> MKKILIVSFLGKGRYYETFYYSIEHSEKMVKKRLSPLANAILEKENGNDVEIIFFVTNEVKNEFLYDENNEYAKNILNELNEIKNYGIKVSYRDIPKGKNYEELEIIMEEIEKLLLDFKGNKVIFDLTHGLR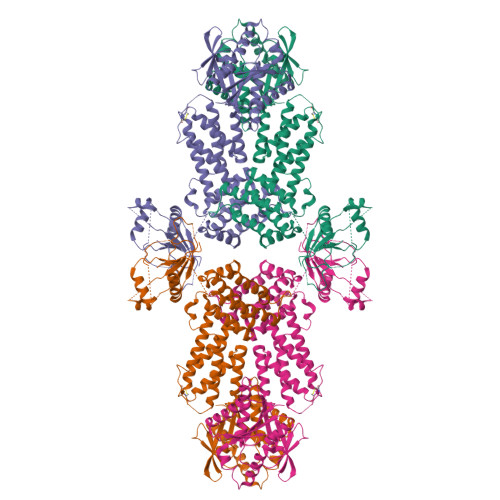HMAIFTSSTVFYFKNLMEKANKLEMKIVYGAYEIGEEIEKNLKKVPILDITQTLELSDLTIALEEFERYGITERMIIVLKNIQKIVAKNKLCNLNELKFSSLSRELKLFEELLKIPSPPEKIANSIYKINDILESSIREFKLCSKNSENLFFIKPIQKFLVDFQKIVLEKLPLDKKINKYSNIATLEKVEFMKNIIKLLINWKMYSEAVIHLRELLIDIKLIENGKYFYYNNKDFREKYWMYSYNIVDTKDKELPKKIEELLKNVKGWRNSVAHGGRANTSINQKTLEENLENALSMIDEILLSMKDLKVNSKKIYLLNSTIMPIPKDNQEGKFYILKLTKNEFKVILENAIKDDVLDSAIGHESVIEFIKDKFELTVPLKRKEIYFEKGESALVIKLEKRPEEGKIYTKEEMDFMEENNLIGYYYIYREG>MSKPQPIAAANWKCNGSQQSLSELIDLFNSTSINHDVQCVVASTFVHLAMTKERLSHPKFVIAAQNAIAKSGAFTGEVSLPILKDFGVNWIVLGHSERRAYYGETNEIVADKVAAAVASGFMVIACIGETLQERESGRTAVVVLTQIAAIAKKLKKADWAKVVIAYEPVWAIGTGKVATPQQAQEAHALIRSWV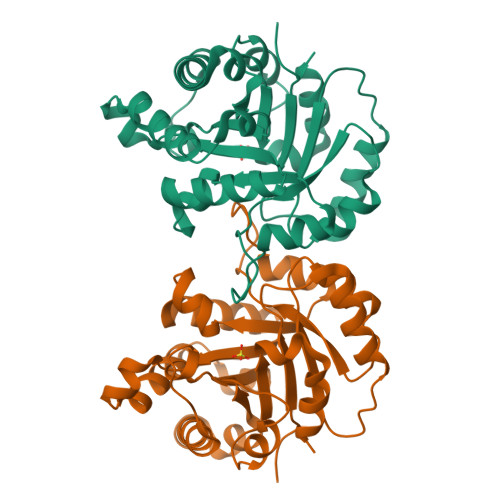SSKIGADVAGELRILYGGSVNGKNARTLYQQRDVNGFLVGGASLKPEFVDIIKATQ[2x]>MAIPAFHPGELNVYSAPGD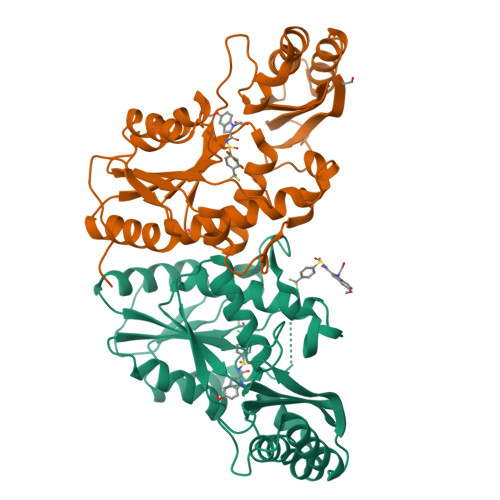VADVSRALRLTGRRVMLVPTMGALHEGHLALVRAAKRVPGSVVVVSIFVNPMQFGAGGDLDAYPRTPDDDLAQLRAEGVEIAFTPTTAAMYPDGLRTTVQPGPLAAELEGGPRPTHFAGVLTVVLKLLQIVRPDRVFFGEKDYQQLVLIRQLVADFNLDVAVVGVPTVREADGLAMSSRNRYLDPAQRAAAVALSAALTAAAHAATAGAQAALDAARAVLDAAPGVAVDYLELRDIGLGPMPLNGSGRLLVAARLGTTRLLDNIAIEIGTFAGTDRPDGYR[2x]4-nitrophenyl beta-D-glucopyranosiduronic acid | C12 H13 N O9 | 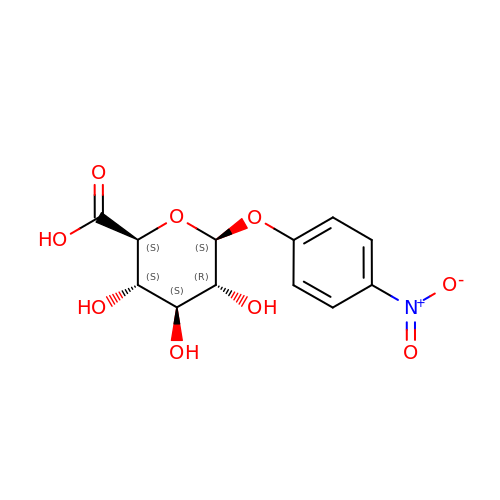QSUILVWOWLUOEU-GOVZDWNOSA-N> MSFTNVNYPASDGTVIFTEEQEALVVQSWNVMKKNSAELGLKLFLKIFEIAPTAKKMFSFVRDSDVPLEQNQKLKGHAMSVFVMTCKSAAQLRKAGKVTFGESSLKHMGSVHLKYGVVDEHFEVTRFALLETIKEAVPEMWSPEMKNAWAEAFNHLVAAIKAEMQRLSTQP

Phytoglobins (Pgbs) are plant-originating heme proteins of the globin superfamily with varying degrees of hexacoordination. Pgbs have a conserved cysteine residue, the role of which is poorly understood. Class 1 Pgbs are distinguished by a weak hexacoordination (KH ≈ 2) compared to Class 2 Pgbs (KH ≈ 100). Due to the very high O2 avidity of Class 1 Pgbs, these proteins generate a tight and slow binding of O2 well suited for O2-dependent nitric oxide (NO) scavenging in low O2-containing environments.

After purification, the two phytoglobins, WT and Cys86Ala, were successfully crystallized. The conditions for crystallization differed slightly, indicating minor differences in the surface properties of the two proteins. The monomers in the dimers showed antiparallel orientation, with the heme groups at the opposite ends of the dimers. In the elucidated WT protein, the distance between the conserved cysteine and the heme iron was 17.3 Å. This can in a first glance be viewed as remote. However, it is well within the 19 Å distance limit that enables electron transfer on ms timescale. When the active center of BvPgb was investigated in more detail, one Tyr residue close to the heme group could easily be identified in position 115, with a distance of 9.24 Å from the heme iron. Therefore, it is plausible that these two residues, Tyr 115 and Cys 86, are both involved in maintaining the redox stability of the iron. Undoubtedly, the conserved cysteine present has a protective role against autoxidation and may be involved in direct electron transfer from the heme iron, affecting the oxidation state.> AGMDVRESISLQNQVSMNLAKHVITTVSQNSNVIFSPASINVVLSIIAAGSAGATKDQILSFLKFSSTDQLNSFSSEIVSAVLADGSANGGPKLSVANGAWIDK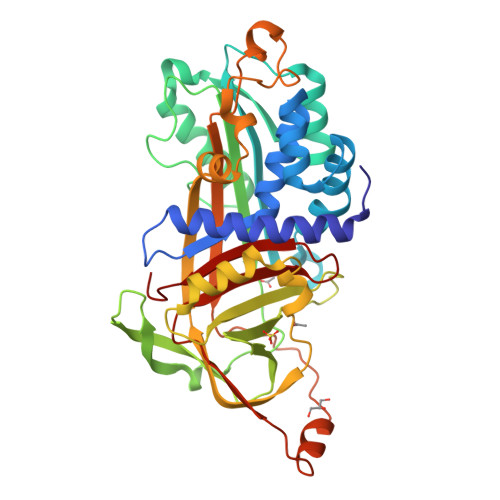SLSFKPSFKQLLEDSYKAASNQADFQSKAVEVIAEVNSWAEKETNGLITEVLPEGSADSMTKLIFANALYFKGTWNEKFDESLTQEGEFHLLDGNKVTAPFMTSKKKQYVSAYDGFKVLGLPYLQGQDKRQFSMYFYLPDANNGLSDLLDKIVSTPGFLDNHIPRRQVKVREFKIPKFKFSFGFDASNVLKGLGLTSPFSGEEGLTEMVESPEMGKNLCVSNIFHKACIEVNEEGTEAAAASAGVIKLRGLLMEEDEIDFVADHPFLLVVTENITGVVLFIGQVVDPLH>[2x]GSHMRSRRVDVMDVMNRLILAMDLMNRDDALRVTGEVREYIDTVKIGYPLVLSEGMDIIAEFRKRFGCRIIAAFKVADIPETNEKICRATFKAGADAIIVHGFPGADSVRACLNVAEEMGREVFLLTEMSHP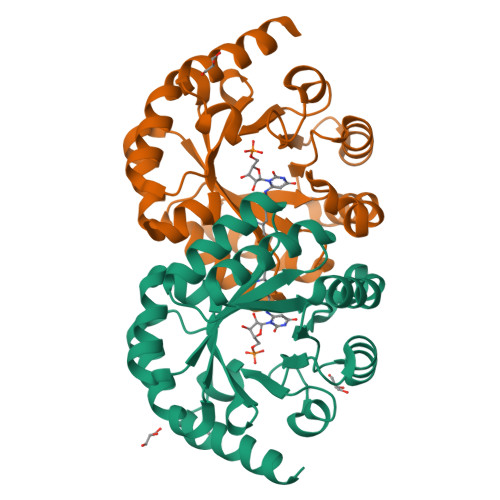GAEMFIQGAADEIARMGVDLGVKNYVGPSTRPERLSRLREIIGQDSFLISPGVGAQGGDPGETLRFADAIIVGRSIYLADNPAAAAAGIIESIKDLRIPEDPAANKARKEAELAAATAEQ>MKVEEILEKALELVIPDEEEVRKGREAEEELRRRLDELGVEYVFVGSYARNTWLKGSLEIDVFLLFPEEFSKEELRERGLEIGKAVLDSYEIRYAEHPYVHGVVKGVEVDVVPCYKLKEPKNIKSAVDRTPFHHKWLEGRIKGKENEVRLLKGFLKANGIYGAEYKVRGFSGYLCELLIVFYGSFLETVKNARRWTRRTVIDVAKGEVRKGEEFFVVDPVDEKRNVAANLSLDNLARFVHLCREFMEAPSLGFFKPKHPLEIEPERLRKIVEERGTAVFAV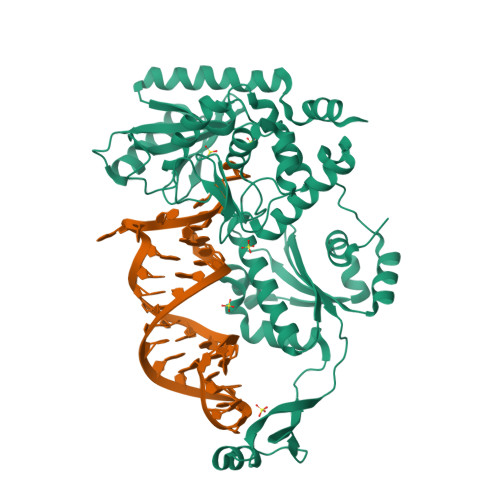KFRKPDIVDDNLYPQLERASRKIFEFLERENFMPLRSAFKASEEFCYLLFECQIKEISRVFRRMGPQFEDERNVKKFLSRNRAFRPFIENGRWWAFEMRKFTTPEEGVRSYASTHWHTLGKNVGESIREYFEIISGEKLFKEPVTAELCEMMGVKDSNSSSVDKLAAALEHHHHHH[4x]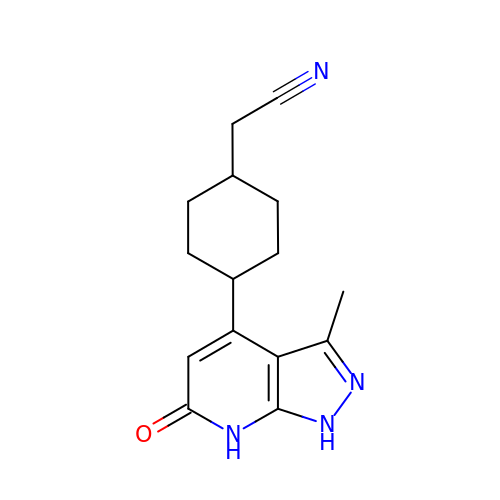2-[4-(3-methyl-6-oxidanylidene-1,7-dihydropyrazolo[3,4-b]pyridin-4-yl)cyclohexyl]ethanenitrile | C15 H18 N4 O | ZPCWQNHNXIMUEY-XYPYZODXSA-N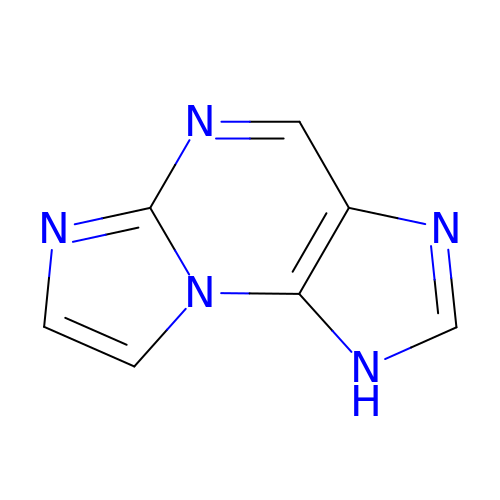N,2,3-etheno-2-aminopurine | C7 H5 N5 | DFRVZUMYUNINCB-UHFFFAOYSA-N>[2x]GSPQLRQVGQIIRVPARMAATLILEPAGRCCWDEPVRIAVRGLAPEQPVTLRASLRDEKGALFQAHARYRADTLGELDLERAPALGGSFAGLEPMGLLWALEPEKPLVRLVKRDVRTPLAVELE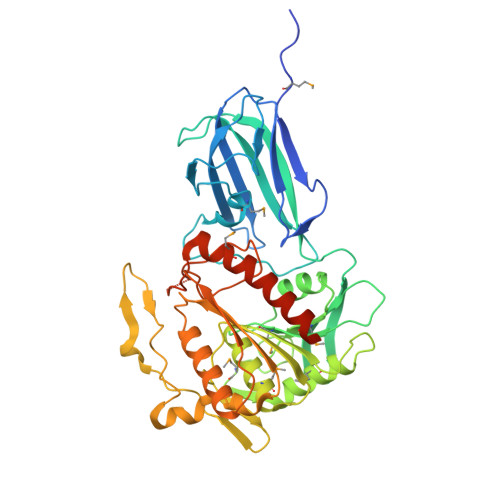VLDGHDPDPGRLLCQTRHERYFLPPGVRREPVRVGRVRGTLFLPPEPGPFPGIVDMFGTGGGLLEYRASLLAGKGFAVMALAYYNYEDLPKTMETLHLEYFEEAMNYLLSHPEVKGPGVGLLGISKGGELCLSMASFLKGITAAVVINGSVANVGGTLRYKGETLPPVGVNRNRIKVTKDGYADIVDVLNSPLEGPDQKSFIPVERAESTFLFLVGQDDHNWKSEFYANEACKRLQAHGRRKPQIICYPETGHYIEPPYFPLCRASLHALVGSPIIWGGEPRAHAMAQVDAWKQLQTFFHKHLGGHEGTIPSKVLEHHHHHH N-(2-ethylphenyl)-2-(3H-imidazo[4,5-b]pyridin-2-ylsulfanyl)acetamide | C16 H16 N4 O S | 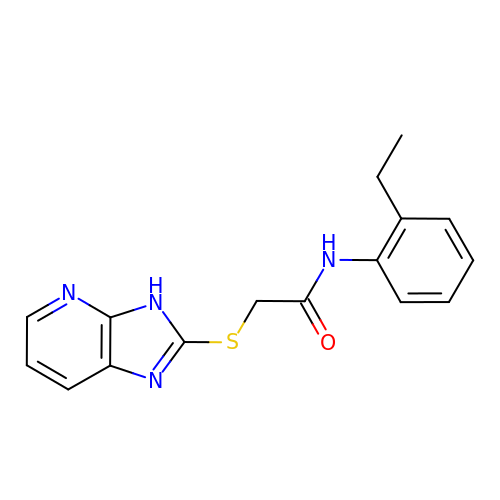LGTSSAOGGPBTGN-UHFFFAOYSA-N> MGTIPKPTLWAEPDSVITQGSPVTLSCQGSLEAQEYRLYREKKSASWITRIRPELVKNGQFHIPSITWEHTGRYGCQYYSRARWSELSDPLVLVMTGAYPKPTLSAQPSPVVTSGGRVTLQCESQVAFGGFILCKEGEDEHPQCLNSQPHARGSSRAIFSVGPVSPNRRWSHRCYGYDLNSPYVWSSPSDLL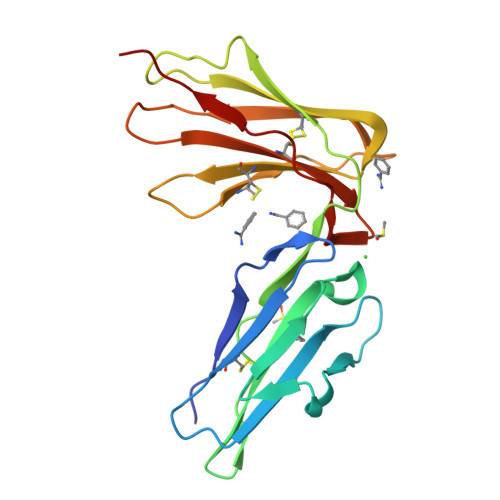ELLVPG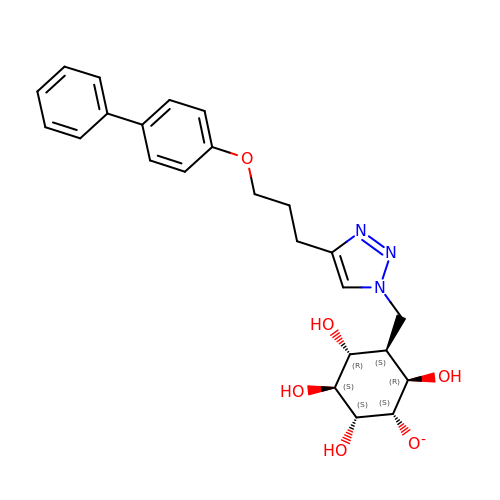(1~{S},3~{S},4~{R},6~{R})-2,3,4,6-tetrakis(oxidanyl)-5-[[4-[3-(4-phenylphenoxy)propyl]-1,2,3-triazol-1-yl]methyl]cyclohexan-1-olate | C24 H28 N3 O6 | IXNAMNDUIMARJW-WVYLNQBTSA-N~{N}-[(1~{S})-1-(1~{H}-benzimidazol-2-yl)-4-(2-fluoranylethanimidoylamino)butyl]-4-phenyl-benzamide | C26 H26 F N5 O | 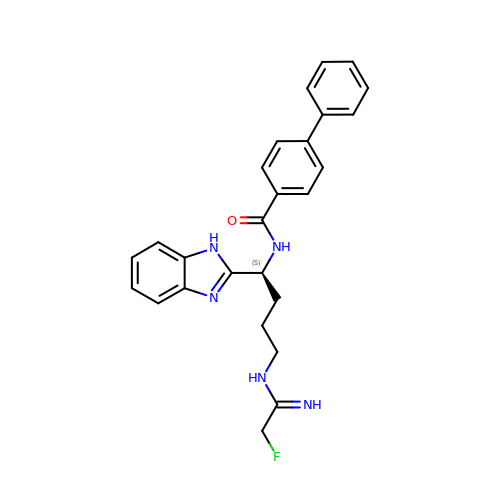YLSHDLCSANAKPH-QHCPKHFHSA-N> T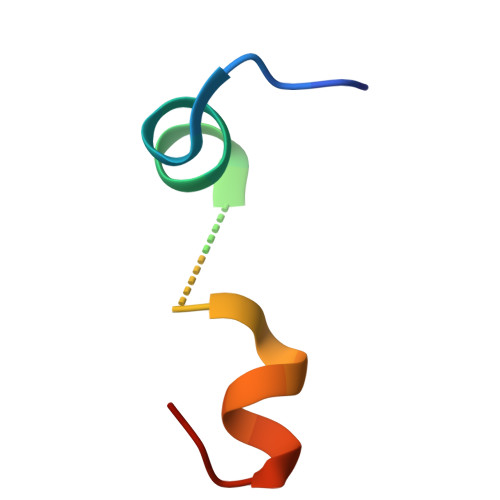VFTSWEEYLDWVGSGDLMPWNLVRIGLLR> GPGGRMGKEVGNLLLENSQLLETKNALNVVKNDLIAKVDQLSGEQEVLKGELEAAKQAKVKLENR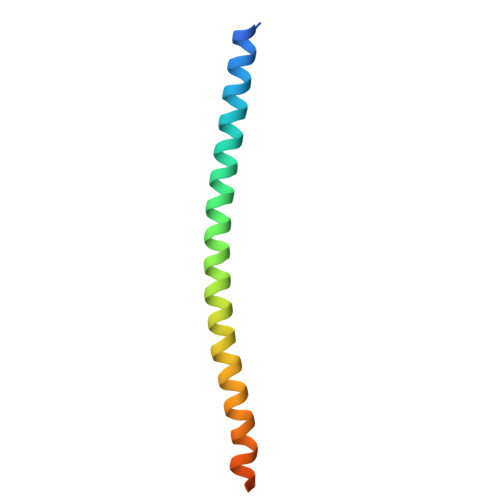IKELEEELKR The 2-methylcitric acid cycle (2-MCC) is widely distributed route of propionate catabolism in microorganisms. That is, some prp operons lack the 2-methylcitrate dehydratase prpD, but rather contain two other genes, acnD and prpF. AcnD has aconitase-like activity, whilst PrpF has aconitate isomerase activity. That is, in organisms that use the AcnD/PrpF enzymes instead of PrpD, 2-methylcitrate is dehydrated by AcnD to 4-methyl-cis-aconitate, which is then isomerized to 2-methyl-cis-aconitate by PrpF, and rehydrated to 2-methylisocitrate by aconitases.

Previous crystallographic data identified residues C107 and K73 in the active site of SoPrpF as likely to be involved in catalysis. In contrast, none of the variants with substitutions at residue K73 supported growth under either condition suggestive of proteins that either lacked catalytic activity or were misfolded. To further understand the roles of residues K73 and C107, we solved the three-dimensional crystal structure of Apo-SoPrpFK73E, which crystallized in space group P21 with cell dimensions a = 51.8 b = 103.4 c = 78.1 Å, and contained two monomers per asymmetric unit. SoPrpF assembles to form a homodimer and buries 2400Å2 of surface area per monomer, which represents 15% of each monomer’s total surface area. While the SoPrpFK73E variant structure can be superposed closely with both the apo-PrpFWT and trans-aconitate bound structures with rms differences of 0.6 Å and 0.4 Å over 385 α-carbon respectively, an alignment of the N-terminal domains from residues 5–185 reveals that the C-terminal domain of the SoPrpFK73E structure rotates into a more open conformation. The C-terminal domain rotates ~4.4° between the extremes provided by the apo (closed) and aconitate (open) bound forms. A comparison of the three structures showed that the trans-aconitate bound structure was in the most open conformation, while the SoPrpFK73E structure was intermediate and the apo-SoPrpFWT structure was in the most closed conformation. Similarly, a malonate molecule derived from the crystallization solution was bound in the active site of the SoPrpFK73E structure. Because malonate is larger than glycerol and smaller than trans-aconitate, the C-terminal domain adopted an intermediary conformation. Attempts to obtain substrate complexed SoPrpFK73E crystals by co-crystallization or soaking into apo crystals with either trans-aconitate or 2-methylcitrate were not successful. This difficulty in co-crystallization was not surprising since binding of trans-aconitate into the SoPrpFK73E active site would position a substrate carboxyl moiety within 3 Å of the new glutamate carboxyl group of SoPrpFK73E variant, thus creating an unfavorable interaction.

>GASSNKLFPPQIKVAATYMRGGTSKGVFFRLQDLPEAAQVPGPARDALLLRVIGSPDPYAKQIDGMGGATSSTSETVILSHSSKANHDVDYLFGQVSIDKPFVDWSGNCGNLTAAVGAFAISNGLIDAARIPRNGVCTVRIWQANIGKTIIAHVPITDGAVQETGDFELDGVTFPAAEVQIEFMNPAADDDGEGGCMFPTGNLVDVLEVPGIGRFNATMINAGIPTIFINAEDLGYTGTELQDDINSDNAALAKFETIRAHGALRMGLIKHIDEAASRQHTPKIAFVAPPKSYASSSGKTVAAEDVDLLVRALSMGKLHHAMMGTAAVAIGTAAAIPGTLVNLAAGGGEKEAVRFGHPSGTLRVGAQAVQENGEWTVIKAIMSRSARVLMEGFVRVPKP[2x]>MATPHINAQMGDFADVVLMPGDPLRAKYIAENFLDNAVQVCDVRNMFGYTGTYKGRKISVMGHGMGIPSCSIYVTELIKDYGVKKIIRVGSCGAVNEGIKVRDVVIGMGACTDSKVNRIRFKDHDFAAIADYKMVKAAEEAAKARGIDVKVGNLFSAELFYTPDPSMFDVMDKYGIVGVEMEAAGIYGVAAEYGAKALAICTVSDHIKTGEQTTSEERQNTF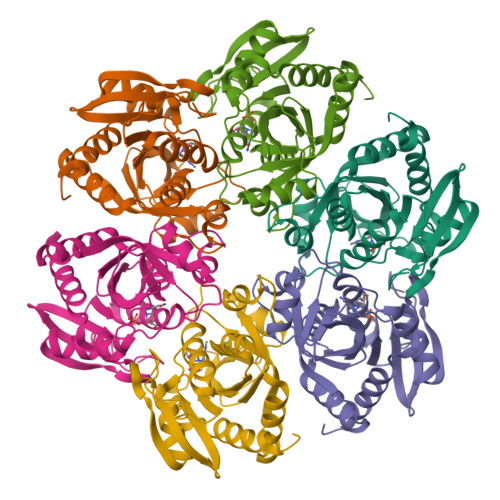NEMIEIALDSVLIGDQAGY[12x]> NLQNIIYNPVIPFVGTIPDQLDPGTLIVIRGHVPSDADRFQVDLQNGSSMKPRADVAFHFNPRFKRAGCIVCNTLINEKWGREEITYDTPFKREKSFEIVIMVLKDKFQVAVNGKHTLLYGHRIGPEKI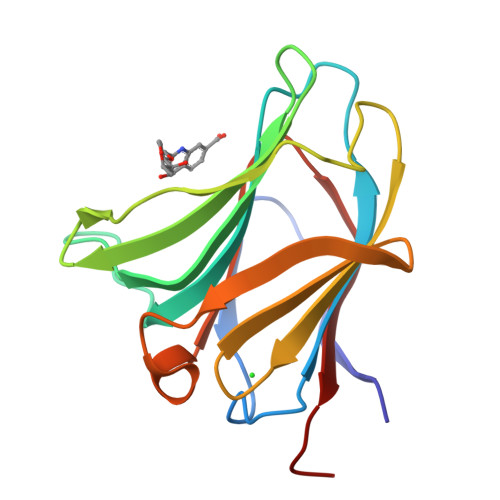DTLGIYGKVNIHSIGFSFSSD;> NNLQNIIYNPVIPFVGTIPDQLDPGTLIVIRGHVPSDADRFQVDLQNGSSMKPRADVAFHFNPRFKRAGCIVCNTLINEKWGREEITYDTPFKREKSFEIVIMVLKDKFQVAVNGKHTLLYGHRIGPEKIDTLGIYGKVNIHSIGFSFSSD>[2x]MRGSHHHHHHGMASHMATEQTAIT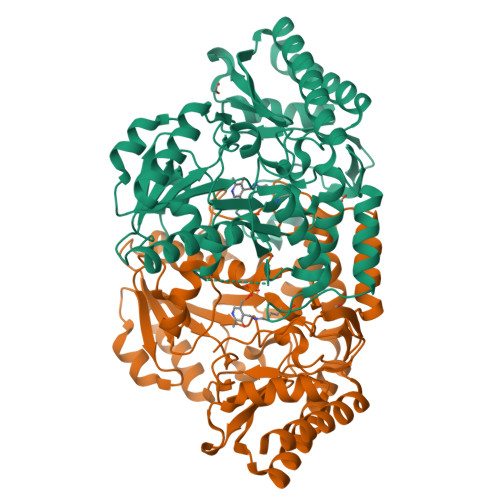RATFDEVILPVYAPADFIPVKGKGSRVWDQQGKEYIDFAGGIAVTALGHCHPALVEALKSQGETLWHTSNVFTNEPALRLGRKLIDATFAERVLFMNSGTEANETAFKLARHYACVRHSPFKTKIIAFHNAFHGRSLFTVSVGGQPKYSDGFGPKPADIIHVPFNDLHAVKAVMDDHTCAVVVEPIQGEGGVQAATPEFLKGLRDLCDEHQALLVFDEVQCGMGRTGDLFAYMHYGVTPDILTSAKALGGGFPVSAMLTTQEIASAFHVGSHGSTYGGNPLACAVAGAAFDIINTPEVLQGIHTKRQQFVQHLQAIDEQFDIFSDIRGMGLLIGAELKPKYKGRARDFLYAGAEAGVMVLNAGADVMRFAPSLVVEEADIHEGMQRFAQAVGKVVA>LPDISRVSHIFFSTKDKKRSDVLDQAKNILSQIRSKKITFEEAVRKYSNDESSKAKNGDLGFLSRGDQNAQNLLGADFVKEVFNFNKGDISSPIASKEGFHIVKVTEKYARPHRDA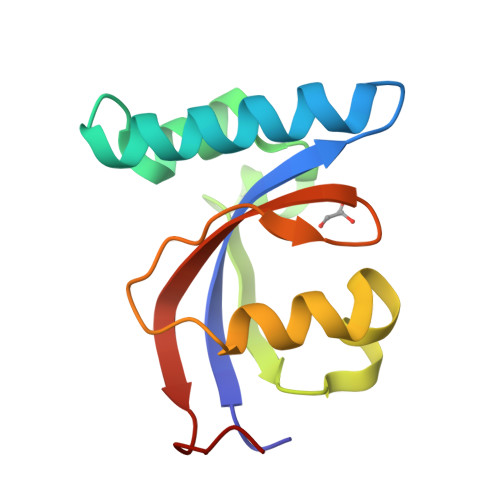[2x]> MKGFSSEDKGEWKLKLDASGNGQAVIRFLPAKTDDALPFAILVNHGFKKNGKWYIETCSSTHGDYDSCPVCQYISKNDLYNTNKTEYSQLKRKTSYWANILVVKDPQAPDNEGKVFKYRFGKKIWDKINAMIAVDTEMGETPVDVTCPWE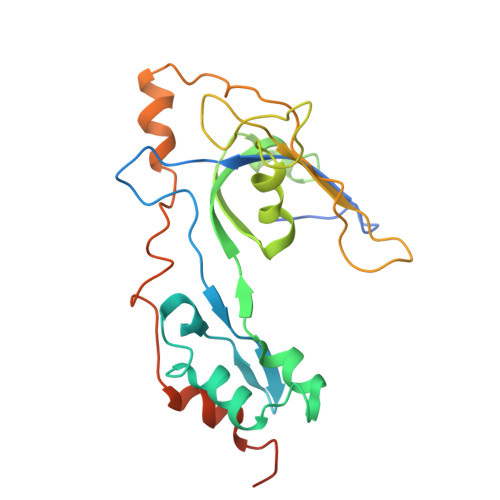GANFVLKVKQVSGFSNYDESKFLNQSAIPNIDDESFQKELFEQMVDLSEMTSKDKFKSFEELNTKFNQVLGTAALGGAAAAAAS> GSAPYASLTEIEHLVQSVCKSYRETCQLRLEDLLRQRSNIFSRE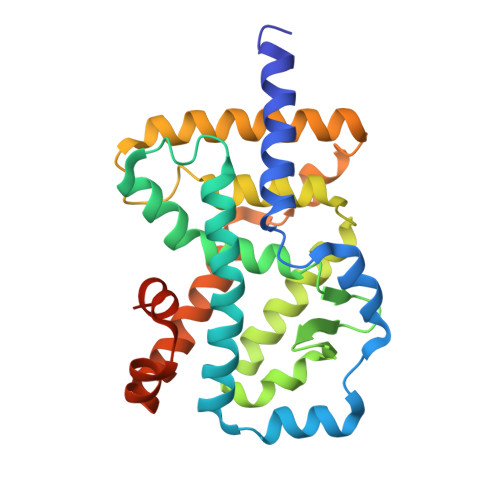EVTGYQRKSMWEMWERCAHHLTEAIQYVVEFAKRLSGFMELCQNDQIVLLKAGAMEVVLVRMCRAYNADNRTVFFEGKYGGMELFRALGCSELISSIFDFSHSLSALHFSEDEIALYTALVLINAHRPGLQEKRKVEQLQYNLELAFHHHLCKTHRQSILAKLPPKGKLRSLCSQHVERLQIFQHLHPIVVQAAFPPLYKELFSTETESPVGLSK> MKYLLPTAAAGLLLLAAQPAMAMDSSGLEVLFQGPGSTSAQAPPVRRLPARFGVEQVRELASRDTRQGVGAGGIAWAISELDLAPVYLNFAENSHLMVTGRRECGRTTTLATIMSEIGRLYAPGASSAPPPAPGRPSAQVWLVDPRRQLLTALGSDYVERFAYNLDGVVAMMGELAAALAGREPPPGLSAEELLSRSWWSGPEIFLIVDDIQQLPPGFDSPLHKAVPFVNRAADVGLHVIVTRTFGGWSSAGSDPMLRALHQANAPLLVMDADPDEGFIRGKMKGGPLPRGRGLLMAEDTGVFVQVAATEVRRLEHHHHHH

EccC, the motor subunit of T7SS, is essential to assemble a stable membrane complex for the secretion process. It contains a two-pass transmembrane domain, an unknown function domain (DUF), and three Fts-SpoIIIE-like ATPase domains (ATPase1, ATPase2, and ATPase3). In this study, we have provided high-resolution crystal structures of ATPase3 domains of EccC proteins from Mtb, all in complex with ATP. In our structures, ATP and a magnesium ion bind to the nucleotide-binding site in a similar manner.

To explain structure-function differences amongst EccC-ATPase3 domains, the crystal structures of Mtb ATPase3 from ESX-2, -3, -5 were determined at 2.20 Å, 1.97 Å and 2.00 Å resolution, respectively. Though the sequence identities are only 20%~30% amongst the four ATPase3 domains, their atomic structures can be superimposed and have r.m.s.d. values in the range 0.99~2.02 Å by comparing Cɑ atom pairs. The second is the loop connecting ɑ1 and β4 (V2), which is extremely long in EccC5-ATPase3. Here, our structural data showed that the recognition pocket in each EccC-ATPase3 is different. The signal binding pocket of MtEccC3-ATPase3 is much wider than MtEccCb1-ATPase3; the pocket of MtEccC5-ATPase3 is much flatter while MtEccC2-ATPase3 has a shallow recognition pocket. Thus, a hexameric model for EccCb1-ATPase3 can be proposed based on the hexamer structure of FtsK ATPase domain through superposition. Indeed, this is similar to what we observed in the packing of our EccC5-ATPase3 crystal structure which has six-fold screw axis symmetry. Similar to FtsK, the protruding segment between ɑ2 and β5 interacts with the loop between β4 and ɑ2 of the neighboring subunit. Such an interaction mode can also be observed in the helical packing of EccC5-ATPase3.>[2x]GSHMASMTGGQQMGRGSTLSEYVQDFLNHLTEQPGSFETEIE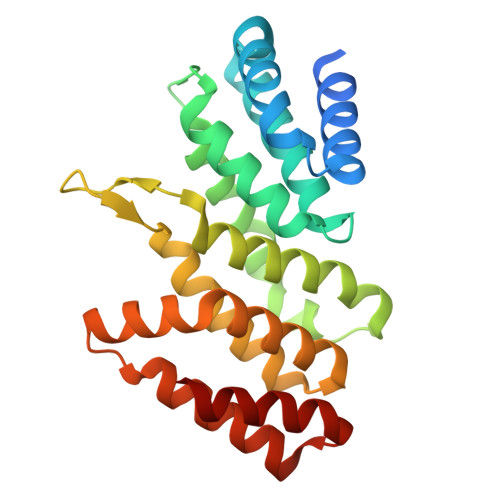QFAETLNGCVTTDDALQELVELIYQQATSIPNFSYMGARLCNYLSHHLTISPQSGNFRQLLLQRCRTEYEVKDQAAKGDEVTRKRFHAFVLFLGELYLNLEIKGTNGQVTRADILQVGLRELLNALFSNPMDDNLICAVKLLKLTGSVLEDAWKEKGKMDMEEIIQRIENVVLDANCSRDVKQMLLKLVELR Cyclodipeptide synthases (CDPS) are a family of tRNA dependant enzymes that synthesise cyclic dipeptides using two aminoacylated tRNA (aa-tRNA) as substrates. Here, we investigated a CDPS from Bacillus thermoamylovorans (BtCDPS), a cLL-synthesising enzyme that utilises Leu-tRNALeu as a substrate, and is predicted to be part of the biosynthetic machinery involved in pulcherrimin biosynthesis. The aminoacyl moiety of tRNA is transferred onto the conserved active site serine residue (S33 in BtCDPS), forming an aminoacyl-enzyme intermediate. This intermediate then reacts with a second aa-tRNA to form a dipeptidyl-enzyme intermediate, which undergoes intramolecular cyclisation aided by a conserved tyrosine residue to form a cyclic dipeptide.

The DBE moiety sits in the P2 pocket and the nitro-groups H-bonds with S33, Y199, S152 and interestingly to R153, which we speculated would interact with the AMP 5′-phosphate group of aa-tRNA substrates. To validate the docking experiment and test the importance of R153 to reactivity and active site architecture, we produced the mutant R153A (BtCDPSR153A). Structurally BtCDPSR153A is extremely similar to the WT BtCDPS and BtCDPSS33C. However, activity with both Leu-tRNALeu and Leu-DBE is completely lost, supporting our observation that this residue likely has an important role during catalysis. Besides the loss of enzyme-substrate interactions, the structure of BtCDPSR153A highlights R153 importance in correctly positioning the active site S33 sidechain (ESI†). The conformation of S33 sidechain is rotated by ∼85°, which orientates it to an inward facing position, closer to the sidechain of Y199 (another catalytic residue) to form an alternative H-bond in the structure of BtCDPSR153A when compared to WT BtCDPS (2.8 Å vs. 3.5 Å). Additionally, helix-7 is displaced (<2 Å) in the BtCDPSR153A, due to the absence of R153.

> GMQQVIKDLFYVVPLSRNCEKIYKNKTHILLGISPFNSKFSQNYIHQLIDWSSKNFKNVTVLLAGDEAKNLLEALGTPTTKAERKVRKEIRRHFRFSEEALRKNGREIDIYTFSDFKNNKIYNEVYQNVIYYFEKDEKFRKSCLAMSHDALSSAAKSLNMEDIEITDNMLFHAVKYVLAELPFFLSGASILGYKESVLAYHRPWKLGEKIKNSEFYIKMSDNQGYIILKQIN> MGDVNGDGTINSTDLTMLKRSVLRAITLTDDAKA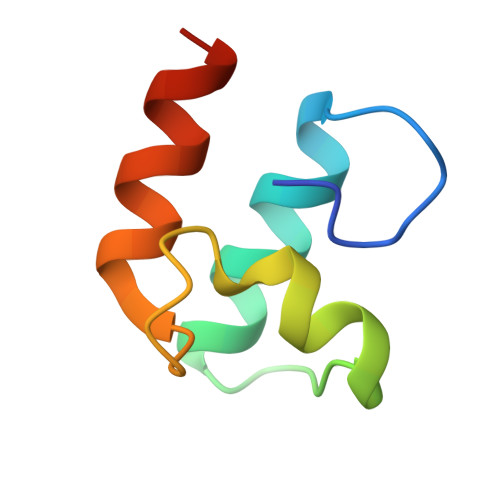RADVDKNGSINSTDVLLLSRYLLRVI> QGPPYPTYP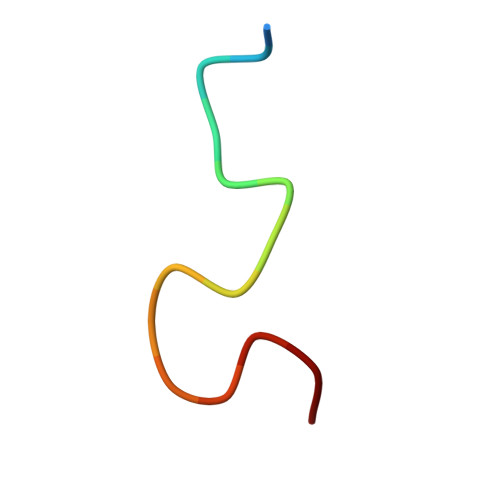GYPGYSQ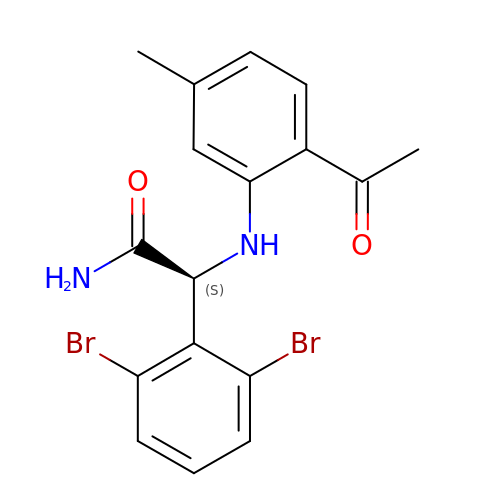(2-ACETYL-5-METHYLANILINO)(2,6-DIBROMOPHENYL)ACETAMIDE | C17 H16 Br2 N2 O2 | FELUFXCUIYHAPB-INIZCTEOSA-N> MSGFDLIIFDCDGVLVDSEIIAAQVE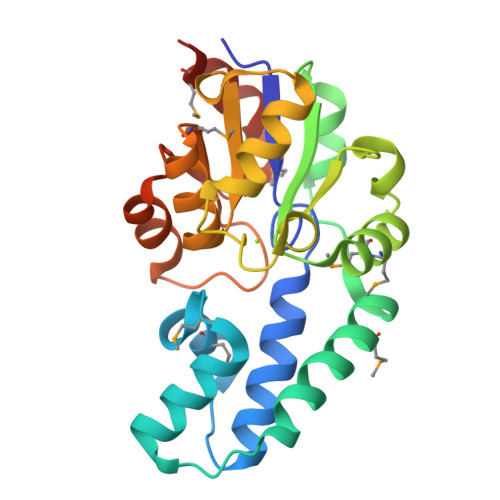SRLLTEAGYPISVEEMGERFAGMTWKNILLQVESEASIPLSASLLDKSEKLLDMRLERDVKIIDGVKFALSRLTTPRCICSNSSSHRLDMMLTKVGLKPYFAPHIYSAKDLGADRVKPKPDIFLHGAAQFGVSPDRVVVVEDSVHGIHGARAAGMRVIGFTGASHTYPSHADRLTDAGAETVISRMQDLPAVIAAMAEWEGAF To elucidate the molecular features encoded by these conserved elements, we solved the crystal structures of Arabidopsis thaliana SOBER1 and Zea mays B6T1C9, each representing a different clade in the phylogenetic tree. Both proteins fold into a canonical α/β hydrolase architecture and superpose with a root-mean-square deviation (RMSD) of atomic positions of 1.54 Å over 210 amino acid residues. We found that a loop constituting the hydrophobic tunnel lid is the major component determining substrate turnover rate and substrate specificity.

To test for the importance of L63 for deacetylation, we constructed a L63A mutant of AtSOBER1 and analyzed its structural and biochemical properties. While wild type AtSOBER1 features a shallow binding groove for the acetate, with a protein surface provided by the side chain of L63, the crystal structure of the L63A mutant showed a massively changed surface, with the hydrophobic tunnel now opened up right behind the active site. In addition, longer substrates were able to enter the tunnel, as demonstrated by higher affinities to pNP butyrate (C4), valerate (C5) and hexanoate (C6). Furthermore, we tested the L63A mutant in tobacco leaves and found the protein to be compromised in AvrBsT-elicited HR repression. The structural information we obtained allowed us to create a mutant (AtSOBER1 L63A), with impaired ability to deacetylate, but is still a functional enzyme with increased activity on longer substrates. In agreement, this mutant protein is compromised in suppression of HR in planta. Taken together with the structural and biochemical data we obtained, this highly suggests deacetylation as the underlying reaction for HR suppression by SOBER1.

> GPMARTFILWLHGLGDSGPANEPIQTQFKSSELSNASWLFPSAPFNPVTCNNGAVMRSWFDVPEAPFKVGSPIDESSVLEAVKNVHAIIDQEIAEGTNPENVFICGLSQGGALTLASVLLYPKTLGGGAVLSGWVPFTSSIISQFPEEAKKTPILWSHGTDDRMVLFEAGQAALPFLKEAGVTCEFKAYPGLGHSISNKELKYIESWIKRRLKGSSSTCLQLNCLKEMFH>[6x]MHHHHHHQHQHENLYFQGMQTKKNEIWVGIFLLAALLAALFVCLKAANVTSIRTEPTYTLYATFDNIGGLKARSPVSIGGVVVGRVADITLDPKTYLPRVTLEIEQRYNHIPDTSSLSIRTSGLLGEQYLALNVGFEDPELGTAILKDGDTIQDTKSAMVLEDLIGQFLYGSKGDDNKNSGDAPAAAPGNNETTEPVGTTK;>[2x]MLLNALASLGHKGIKTLRTFGRAGLMLFNALVGKPEFRKHAPLLVRQLYNVGVLSMLIIVVSGVFIGMVLGLQGYLVLTTYSAETSLGMLVALSLLRELGPVVAALLFAGRAGSALTAEIGLMRATEQLSSMEMMAVDPLRRVISPRFWAGVISLPLLTVI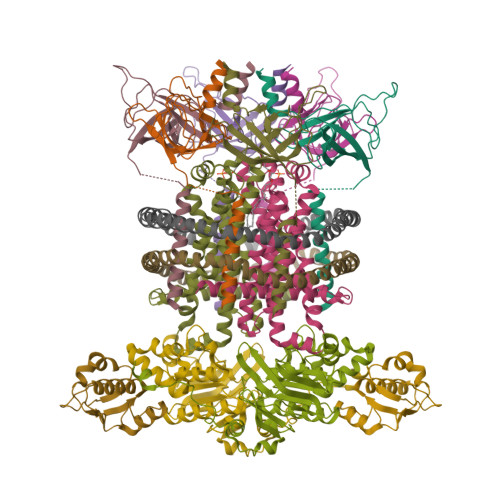FVAVGIWGGSLVGVSWKGIDSGFFWSAMQNAVDWRMDLVNCLIKSVVFAITVTWISLFNGYDAIPTSAGISRATTRTVVHSSLAVLGLDFVLTALMFGN;>MEQSVANLVDMRDVSFTRGNRCIFDNISLTVPRGKITAIMGPSGIGKTTLLRLIGGQIAPDHGEILFDGENIPAMSRSRLYTVRKRMSMLFQSGALFTDMNVFDNVAYPLREHTQLPAPLLHSTVMMKLEAVGLRGAAKLMPSELSGGMARRAALARAIALEPDLIMFDEPFVGQDPITMGVLVKLISELNSALGVTCVVVSHDVPEVLSIADHAWILADKKIVAHGSAQALQANPDPRVRQFLDGIADGPVPFRYPAGDYHADLLPGS[2x];>MSESLSWMQTGDTLALSGELDQDVLLPLWEMREEAVKGITCIDLSRVSRVDTGGLALLLHLIDLAKKQGNNVTLQGVNDKVYTLAKLYNLPADVLPR[2x]> TVGAVALDLDGNLAAATSTGGMTNKLPGCVGSVPLVGAGCYANNASVAVSCTGTGEVFIRALAAYD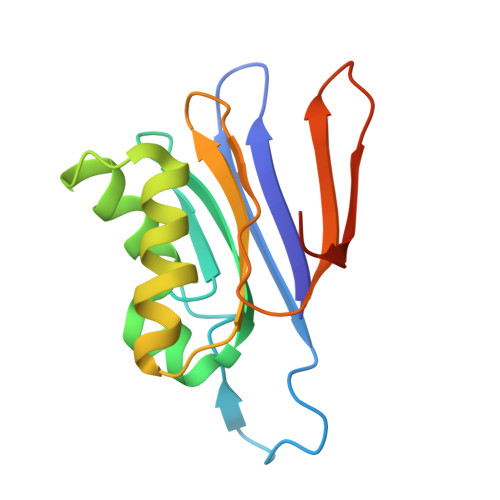IAALMDYGGLSLAEACERVVMEKLPALGGSGGLIAIDHEGNVALPFNTEGMYRAWGYAGDTPTTGIYREKGDTVATQ>EYGDLHLFGPNQRPAPCYDPCEAVLVESIPEGLDFPNASTGNPSTSQAWLGLLAGAHSSLDIASFYWTLTNNDTHTQEPSAQQGEEVLRQLQTLAPKGVNVRIAVSKPSGPQPQADLQALLQSGAQVRMVDMQKLTHGVLATKFWVVDQTHFYLGSANMDWRSLTQVKELGVVMYNCSCLARDLTKIFEAYWFLGQAGSSIPSTWPRFYDTRYNQETPMEICLNGTPALAYLASAPPPLCPSGRTPDLKALLNVVDNARSFIYVAVMNYLPTLEFSHPHRFWPAIDDGLRRATYERGVKVRLLISCWGHSEPSMRAF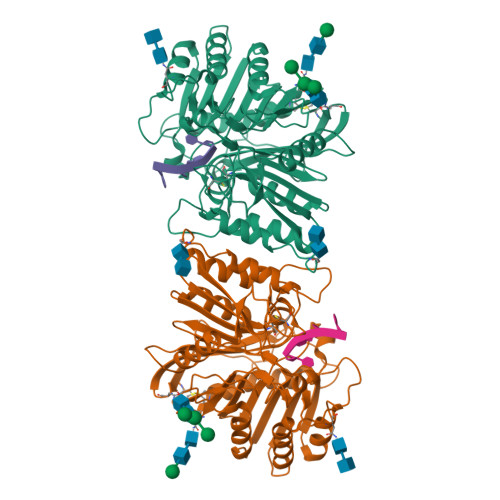LLSLAALRDNHTHSDIQVKLFVVPADEAQARIPYARVNANKYMVTERATYIGTSNWSGNYFTETAGTSLLVTQNGRGGLRSQLEAIFLRDWDSPYSHDLDTSADSVGNACRLLLEVLFQ[2x]> MNCRSEVLEVSVEGRQVEEAMLAVLHTVLLHRSTGKFHYAAAGTYSIGTVGTQDVDCDFIDFTYVRVSSEELDRALRKVVGEFKDALRNSGGDGLGQMSLEFYQKKKSRWPFSDECIPWEVWTVKVHVVALATEQERQICREKVGEKLCEKIINIVEVMNRHEYLPK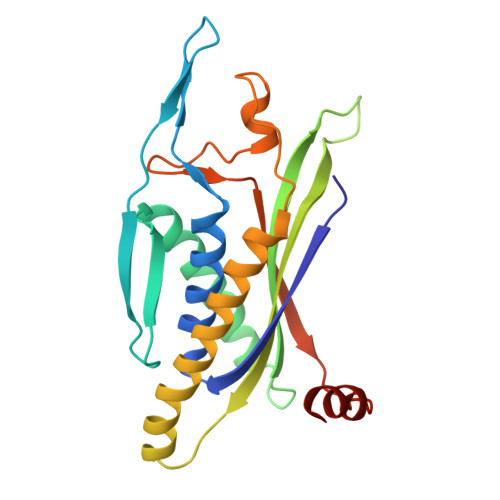MPTQSEVDNVFDTGLRDVQPYLYKISFQITDALGTSVTTTMRRLIKDTLAL>[6x]MLNQELELSLNMAFARAREHRHEFMTVEHLLLALLSNPSAREALEACSVDLVALRQELEAFIEQTTPVLPASEEERDTQPTLSFQRVLQRAVFHVQSSGRNEVTGANVLVAIFSEQESQAAYLLRKHEVSRLDVVNFISHGTRKDEPTQSSDPGSQPNSEEQAGGEERTENFTTNLNQLARVGGIDPLIGREKELERAIQVLCRRRKNNPLLVGESGVGKTAIAEGLAWRIVQGDVPEVMADCTIYSLDIGSLLAGTKYRGDFEKRFKALLKQLEQDTNSILFIDEIHTIIGAGAASGGQVDAANLIKPLLSSGKIRVIGSTTYQEFSNIFEKDRALARRFQKIDITEPSIEETVQIINGLKPKYEAHHDVRYTAKAVRAAVELAVKYINDRHLPDKAIDVIDEAGARARLMPVSKRKKTVNVADIESVVARIARIPEKSVSQSDRDTLKNLGDRLKMLVFGQDKAIEALTEAIKMARAGLGHEHKPVGSFLFAGPTGVGKTEVTVQLSKALGIELLRFDMSEYMERHTVSRLIGAPPGYVGFDQGGLLTDAVIKHPHAVLLLDEIEKAHPDVFNILLQVMDNGTLTDNNGRKADFRNVVLVMTTNAGVRETERKSIGLIHQDNSTDAMEEIKKIFTPEFRNRLDNIIWFDHLSTDVIHQVVDKFIVELQVQLDQKGVSLEVSQEARNWLAEKGYDRAMGARPMARVIQDNLKKPLANELLFGSLVDGGQVTVALDKEKNELTYGFQSAQKHKAEAAH;>ALVPMVIEQTSRGERSFDIYSRLLKERVIFLTGQVEDHMANLIVAQMLFLEAENPEKDIYLYINSPGGVITAGMSIYDTMQFIKPDVSTICMGQAASMGAFLLTAGAKGKRFCLPNSRVMIHQPLGGYQGQATDIEIHAREILKVKGRMNELMALHTGQSLEQIERDTERDRFLSAPEAVEYGLVDSILTHRNRSHHHHHH[7x];> MGKTNDWLDFDQLAEEKVRDALKPPSMYKVILVNDDYTPMEFVIDVLQKFFSYDVERATQLMLAVHYQGKAICGVFTAEVAETKVAMVNKYARENEHPLLCTLEKA

ClpAP, a two-ring AAA+ protease, degrades N-end-rule proteins bound by the ClpS adaptor. AAA+ proteases, such as ClpAP, consist of a hexameric AAA+ unfoldase (for example, ClpA6) and a self-compartmentalized peptidase (for example, ClpP14). Each ClpA subunit has two AAA+ modules, called D1 and D2, that associate in the hexamer to form two stacked rings. Here we present high-resolution cryo-EM structures of Escherichia coli ClpAPS complexes, showing how ClpA pore loops interact with the ClpS N-terminal extension (NTE), which is normally intrinsically disordered.

For example, density for the ClpS NTE was present in both the ClpA D1 and D2 rings in classes I and II, but only in the D1 ring of class III. Loss of D2 pore-1 loop engagement with the ClpS NTE is a major feature distinguishing our class-III structures from classes I and II. Most surprisingly, the D2 pore-1 loops in class III were rotated ~90° compared to their orientation in classes I and II, and the key Tyr540 side chains were tucked in and turned away from the channel. In both class-III subclasses, at least four of the six pore-1 loops were convincingly in the tucked conformation. Three additional features of the class-III D2 ring are noteworthy. Coincident with the pore-1-loop rotation, the ClpA channel in the D2 ring of class III was ~2 Å wider than in classes I and II. Second the D2 rigid-body interface between the small AAA+ domain of subunit E and its neighboring large AAA+ domain in subunit F was broken in class III. Finally, the D2 ring contained ADP in three adjacent subunits in class III, whereas classes I and II contained no more than two ADPs in the D2 ring. Moreover, the portion of the ClpS NTE in the D1 ring of class-III structures is bound in the same fashion as our class-I and class-II structures.> GSTGSMKKTLVAGFAVAALSTGIFAVSNEANAQVTSQNGIILHDDSRMLDHELQYVDVLINPNANPQTKERLKAYFESQGLNTVSEIVQKAKQD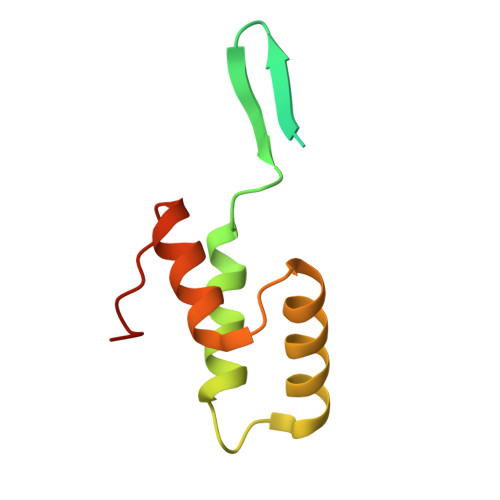GLDTSKYDHLI> VPQDASTKKLSECLK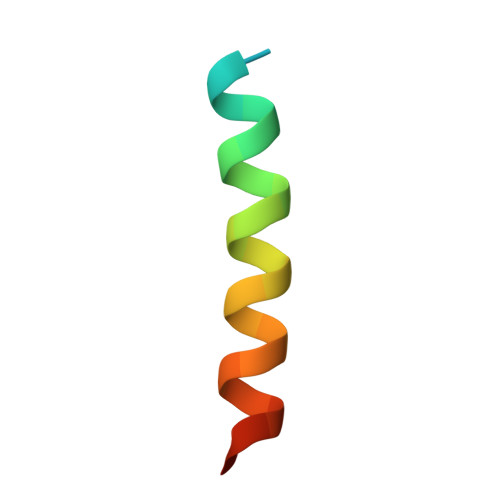RIGDELDSNMELQ>GLTEEQKQEIREAFDLFDTDGSGTIDAKELKVAMRALGFEPKKEEIKKMIADIDKDGSGTIDFEEFLQMMTAKMGERDSR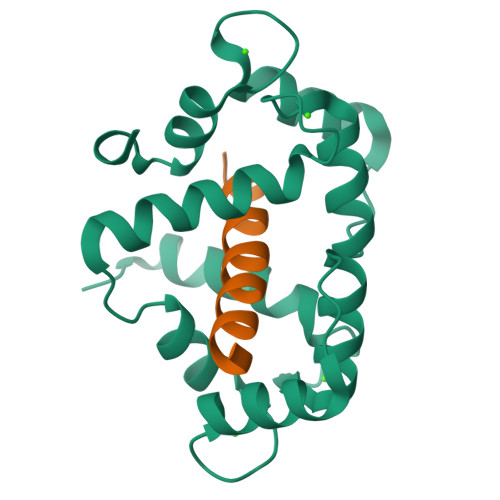EEIMKAFRLFDDDETGKISFKNLKRVAKELGENMTDEELQEMIDEADRDGDGEVNEEEFFRIMKKTSLF[2x];>[2x]KRRWKKNFIAVSAANRFKKISS5-(4-METHOXYPHENOXY)-2,4-QUINAZOLINEDIAMINE | C15 H14 N4 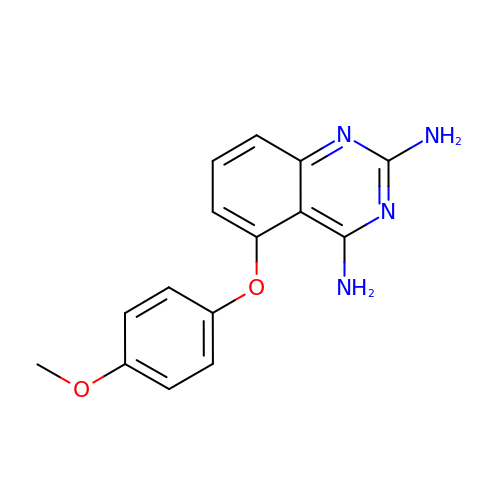O2 | CPZJZAIZIMCJRC-UHFFFAOYSA-N>[2x]MMKPEDVIKEQCARAKVVAELWHGFTGGAPKAALENLVVEFNKAQQGRCVRPVPQGGYRDLSTKIKAAFAAGKVPTMAQAFEANIALYLEAKALL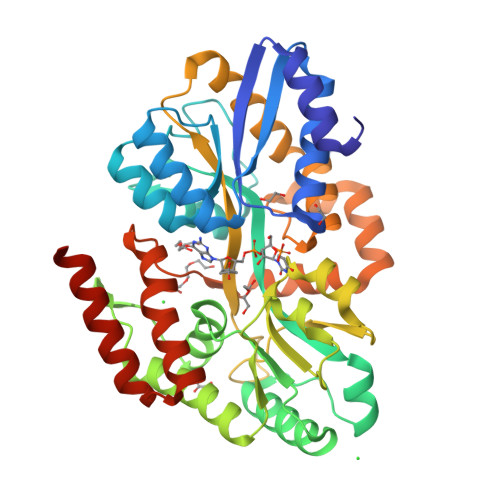PIESLGVKLQGVNLTFLNAVRFGGVVYGVPFNKSIQVLYYNKDLLKKHGVPVPATLEEFVAAAKKLSRAEGGPVYWFQPDASTFAYFFFNLGGSYLKDGKLVLNSKEAVEALTLLQNGVKEGWAKPITSGYINQNLGSGPYAFSVDTSAGYTYYLRAAKFDLGVATLPGRTKGQPGYGLVQGTNLVVFRQASKEEQAVAKDFLEFVLSPRAQAVFATATGYVPVTEGALKDPVYQAYAAENPDYATIVRQSRYAKFEPALAEWEQIRFDILGQAIKEAILNKADPKAALDRAQKLAEDLLSSRTRHHHHHH> MNQIEPGVQYNYVYDEDEYMIQEEEWDRDLLLDPAWEKQQRKTFTAWCNSHLRKAGTQIENIEEDFRNGLKLMLLLEVISGERLPKPDRGKMRFHKIANVNKALDYIASKGVKLVSIGAEEIVDGNVKMTLGMIWTIILRFAIQDISVEETSAKEGLLLWCQRKTAPYRNVNIQNFHTSWKDGLGLCALIHRHRPDLIDYSKLNKDDPIGNINLAMEIAEKHLDIPKMLDAEDIVNTPKPDERAIMTYVSCFYHAFAGAEQAETAANRICKVLAVNQENERLMEEYERLASELLEWIRRTIPWLENRTPEKTMQAMQKKLEDFRDYRRKHKPPKVQEKCQLEINFNTLQTKLRISNRPAFMPSEGKMVSDIAGAWQRLEQAEKGYEEWLLNEIRRLERLEHLAEKFRQKASTHETWAYGKEQILLQKDYESASLTEVRALLRKHEAFESDLAAHQDRVEQIAAIAQELNELDYHDAVNVNDRCQKICDQWDRLGTLTQKRREALERMSERVRNFE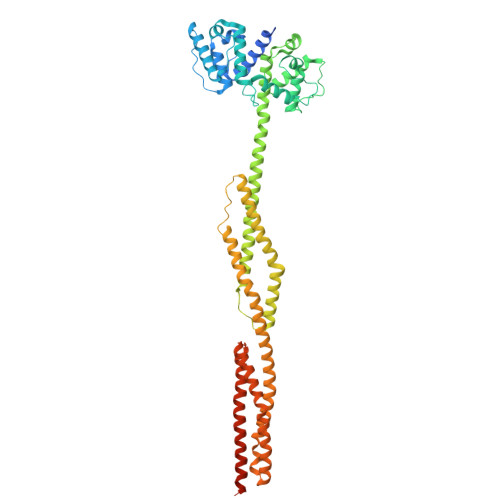DPAANKARKEAELAAATAEQ> ENLMQVYQQARLSNPELRKSAADRDAAFEKINEARSPLLPQLGLGADYTYSNGYRDANGINSNATSASLQLTQSIFDMSKWRALTLQEKAAGIQDVTYQTDQQTLILNTATAYFNVLNAIDVLSYTQAQKEAIYRQLDQTTQRFNV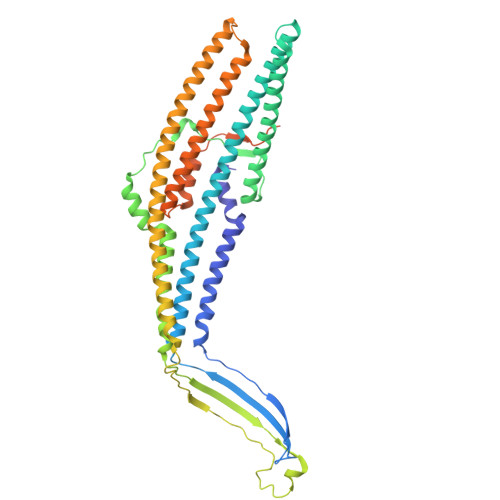GLVAITDVQNARAQYDTVLANELTARNNLDNAVEQLRQITGNYYPELAALNVENFKTDKPQPVNALLKEAEKRNLSLLQARLSQDLAREQIRQAQDGHLPTLDLTASTGISDTSYSGSKTRGAAGTQYDDSNMGQNKVGLSFSLPIYQGGMVNSQVKQAQYNFVGASEQLESAHRSVVQTVRSSFNNINASISSINAYKQAVVSAQSSLDAMEAGYSVGTRTIVDVLDATTTLYNAKQELANARYNYLINQLNIKSALGTLNEQDLLALNNALSKPVSTNPENVAPQTPEQNAIADGYAPDSPAPVVQQTSARTTTSNGHNPFRNDYKDDDDK> MSKRLPPLNALRVFDAAARHLSFTRAAEELFVTQAAVSHQIKSLEDFLGLKLFRRRNRSLLLTE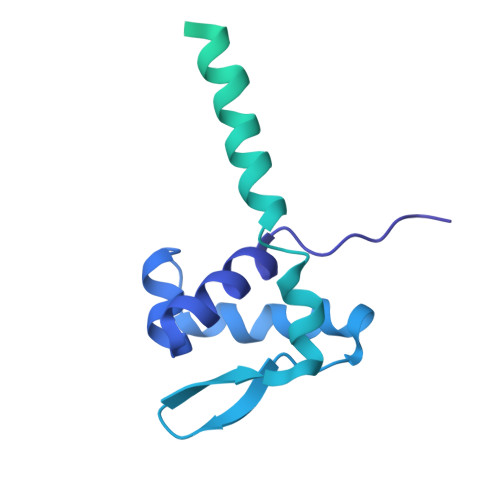EGQSYFLDIKEIFSQLTEATRKLQARSAKGALTVSLLPSFAIHWLVPRLSSFNSAYPGIDVRIQAVDRQEDKLADDVDVAIFYGRGNWPGLRVEKLYAEYLLPVCSPLLLTGEKPLKTPEDLAKHTLLHDASRRDWQTYTRQLGLNHINVQQGPIFSHSAMVLQAAIHGQGVALANNVMAQSEIEAGRLVCPFNDVLVSKNAFYLVCHDSQAELGKIAAFRQWILAKAAAEQEKFRFRYEQ> SGVDDDMACHKIPVEADFLYAYSTAPGYYSWRNSKDGSWFIQSLCAMLKQYADKLEFMHILTRVNRKVAAEFESFSFDATFHAKKQIPCIVSMLTKEL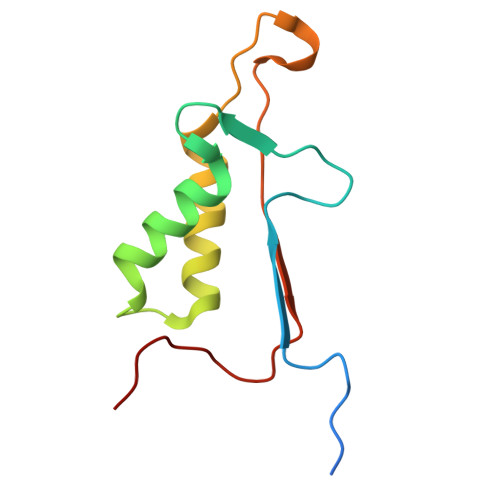YFYHH>MMYRAPKTEKGKESLNKILDASVELIADKGFLSTSINDITSKAGVAYGLFYFYFKSKHDILDEIIRQFNRNMRYYLKTYTQNLDSRIDVEKVGMKKFLEWMNENKKYYKIFIETQVHRPDIYKWHFMKLAERYTTGLSEAMRRGEIINVDPELLSYVLIGIAHMLGKRYVLWSNSGLTLKQQRDLDLIIENMLTPR[6x]

FadRSa, of which we show that it displays structural similarities with bacterial TetR-like FadR regulators, is an archaeal member of the widespread prokaryotic TetR family. Each subunit displays two functional domains: an N-terminal helix-turn-helix (HTH) DNA-binding domain (α1–α3) and a C-terminal domain (α4–α9) of which α8 and α9 stabilize dimerization. The finding that FadRSa represses the Saci_1103-Saci_1126 gene cluster and that it is responsive to acyl-CoA molecules acting as inducers in vitro strongly suggests that intracellularly present acyl-CoA molecules cause a derepression and thus higher transcriptional expression of the gene cluster in vivo.

To further unravel mechanisms of DNA binding by FadRSa, we determined the cocrystal structure of the protein–DNA complex to a resolution of 3.29 Å using a duplex DNA containing the predicted FadRSa binding motif in the control region of the fadRSa gene itself, corresponding to ChIP-seq peak 2. The asymmetric unit contained six FadRSa subunits, organized as three dimers, and two DNA duplex molecules thus representing a nonbiological assembly, although the protein–DNA molecular interactions within this structure are representative of the biologically relevant complexes (see below, DNA-binding stoichiometry of FadRSa). In each FadRSa subunit in the cocrystal structure, residues of the recognition helix α3 and the α2–α3 loop interact with the major groove of DNA with the establishment of an extensive number of contacts. Besides protein–DNA contacts, a weak electrostatic protein–protein contact was also observed between Asn37 residues of FadRSa dimers bound on different sides of the DNA helix. The presence of a G–C bp 11 positions upstream of the symmetrical C–G in the pseudopalindromic site appears to be the sole explanation of the preference of a second FadRSa dimer to establish an interaction with the upstream (left) and not downstream (right) side of the pseudopalindromic site. Based on the cocrystal structure, the G base of this G–C bp in the fadRSa operator can be assumed to be contacted by Gly48 that is crucial for DNA binding with the dimer-of-dimer-complex architecture reflecting that of the architecture of the AB dimer and subunit E of the DE dimer interacting with a single-DNA duplex in the cocrystal structure. A Gly48–guanine interaction and Asn37-mediated protein–protein contacts, of which the latter have never before been observed for bacterial dimer-of-dimer binding TetR-like proteins, assist in the dimer-of-dimer interaction mode.> SSSNYCNQMMKSRNLTKD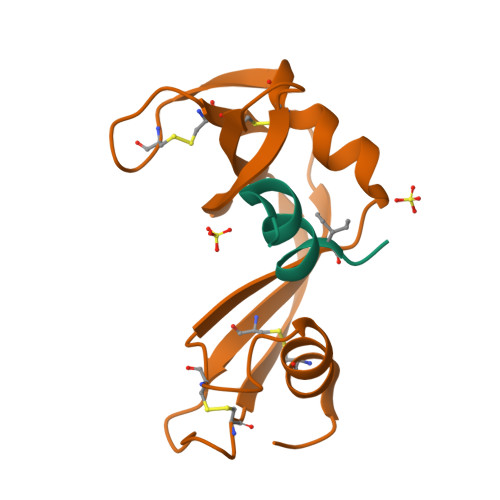RCKPVNTFVHESLADVQAVCSQKNVACKNGQTNCYQSYSTMSITDCRETGSSKYPNCAYKTTQANKHIIVACEGNPYVPVHFDASV;> KETAAAKFERQHVDS One such multienzyme is propionyl-CoA carboxylase (PCC), which catalyzes the carboxylation of propionyl-CoA to form methylmalonyl-CoA, a precursor to the citric acid cycle intermediate succinyl-CoA. Propionyl-CoA carboxylase (PCC) is a multienzyme complex consisting of up to six α-subunits and six β-subunits. The α-subunit of LtPCC contains three domains: a biotin carboxylase (BC) domain, BC-CT mediating (BT) domain, and biotin carboxyl carrier protein (BCCP) domain. The β-subunit is composed of the structurally homologous N-carboxyltransferase (N-CT) and C-carboxyltransferase (C-CT) domains (Huang et al., 2010, Scheffen et al., 2021).

With D3 symmetry, we obtained a map of the LtPCC α6β6 dodecamer at 3.2 Å resolution. As a dodecamer, PCC contains two layers of α-subunits sandwiching a β-homohexamer. Each layer of α-subunits contains three monomeric α-subunits, while the six β-subunits in the β-homohexamer are arranged into a two-layered cylinder. Accordingly, we observed a clear density for biotin next to Lysine 631 of the AMKM motif in the β-subunit active site. There is weak density connecting lysine and biotin, suggesting that some LtPCC assemblies are covalently biotinylated. CoA was not observed at its β-subunit binding site. No interactions exist among LtPCC α-subunits. There are seven hydrogen bonds between α- and β-subunits. Taken together, hydrophobic interactions and hydrogen bonds contribute to the α-β binding site to stabilize the α-subunits onto the β-homohexamer. We found that most endogenous LtPCCs exist as α6β6, and in descending frequency, LtPCC also exhibit oligomeric isoforms with the oligomeric formulae α5β6, α4β6, α3β6, α2β6, α1β6, and α0β6.

>[6x]VLVANRGEIACRVMATCRRLGIKTVAVYSTADEQAKHVKVADESVCIGPPASVESYLCIDKIVDACKKTGAQAVHPGYGFLSENGEFQSALQKNNIVFVGPDAHSIESMGDKIESKRLAQRAGVTCIPGFIGEVKTHEDLLRFAREIGYPVMIKASGGGGGKGMRVAYNDTQCVEYYDMCREEAKAAFHSDKMLVERFIDHPRHIEIQVIADRRGNTVYLPERECSIQRRNQKVIEEAPSVLLDATTRKAMGEEAVAMARAVQYVSAGTVENVVNPQKQFYFLEMNTRLQVEHPITEEITGVDLVEQMLRAAADLPLSITQDDITINGHATECRVYAEDPMKNYFPSIGRLTMYQEPTGAGVRCDSGIIEGSQISVYYDPLICKLSTWGRDRAECIGRMEKALDEYVIRGLRHNICLLRDVVTEPRYRSGSITTNYLQEQYPNGFKKAELTAEEMQLMYEVAACVHLKRERLHYTQGTAPSERQLYLSVGAGQEGETPVYVRYLDDSHFEIGASKHGPFRKMEVVWKASYPIIRVKDGEAETVLQFWGTNEVTYGMQMRGTTFDVNVMSDLQSTLAHFVPITEATTNTKQILSPMPGVIVAIKVQPGQMVVAGEELLTLEAMKMRNKIHAQADGKVKEVKVKLGATVEDNEVLVELE;>PTAAEDLRHKKKRLTAMERVQLFCDPGTFRERDALVEHECHNFGMEKRKVPGDGFITGTGKVFGRPVFLFSHDFTVFGGSLSRTNAAKVVRIMEEAAKIGVPVIGFNDSGGARIHEGVDSLAGYADIFLRNTLFSGVIPQISVIMGPCAGGAVYSPAITDFTFMVETSSYMFVTGPEVVSAVGGKLVTKDELGGPHVHATKSGVSAGTFPNDIVAMAQLRRLYSYLPLSNRDPVPVLPTADERYRDVSSLNTVVPTEVKEAYDMRDVIYPVIDHDSFFEIQPQFAKNIICGFARVEGRSVCIIANQPKVQAGVLDIDSSVKGARMVRFADAFNIPIITFVDVPGFLPGVQQEYGGIIRHGAKLLYAYAEATVPKVTIITRKAYGGAYDVMSSKHLRGDSNYAWPHAEIAVMGAAGACKLLYSKETAEQQAQRIADYEKTFCTPLSAARKGFVDAVIDPSETRMRVCEDLERLARKQLQNPWKKHGNIPL[6x]>MSKVKVAVRVRPMNRREIDLHTKCVVDVEANKVILNPINTNLSKGDARGQPKIFAYDHCFWSMDESVREKYAGQDDVFKCLGENILQNAFDGYNACIFAYGQTGSGKSYTMMGTADQPGLIPRLCSGLFERTQKEENEEQSFKVEVSYMEIYNEKVRDLLDPKGSRQTLKVREHSVLGPYVDGLSKLAVTSYKDIESLMSEGNKSRTVAATNMNEESSRSHAVFKITLTHTLYDVKSGTSGEKVGKLSLVDLAGSERATKTGAA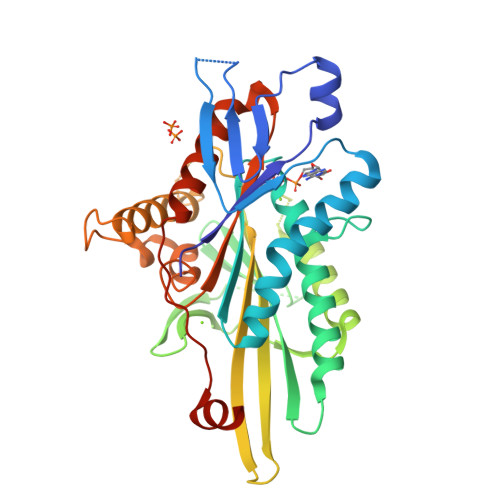GDRLKEGSNINKSLTTLGLVISALADQGAGKNKNKFVPYRDSVLTWLLKDSLGGNSKTAMVATVSPAADNYDETLSTLRYADRAKHIINHAVVNEDPNARIIRDLHHHHHH[3x]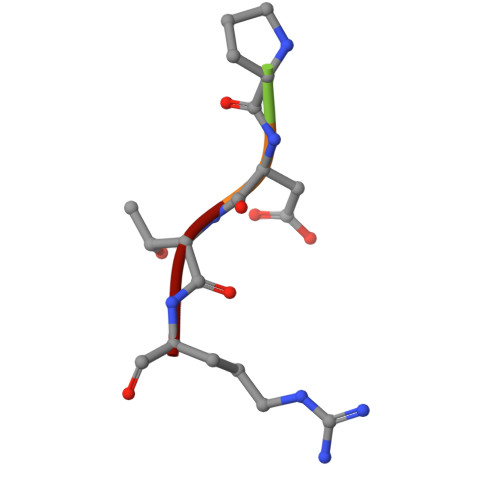> APDTR> MAAECATQRAPGSVVELLGKSYPQDDHSNLTRKVLTRVGRNLHNQQHHPLWLIKERVKEHFYKQYVGRFGTPLFSVYDNLSPVVTTWQNFDSLLIPADHPSRKKGDNYYLNRTHMLRAHTSAHQWDLLHAGLDAFLVVGDVYRRDQIDSQHYPIFHQLEAVRLFSKHELFAGIKDGESLQLFEQSSRSAHKQETHTMEAVKLVEFDLKQTLTRLMAHLFGDELEIRWVDCYFPFTHPSFEMEINFHGEW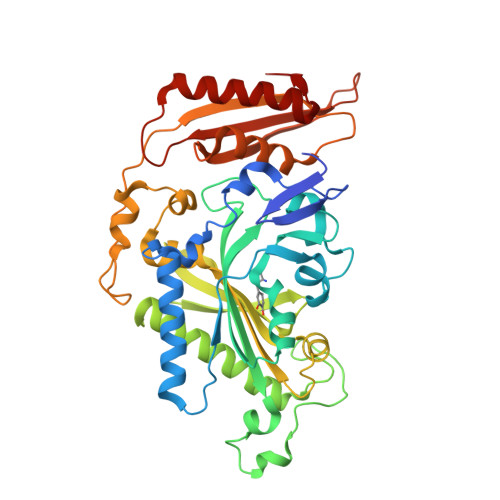LEVLGCGVMEQQLVNSAGAQDRIGWAFGLGLERLAMILYDIPDIRLFWCEDERFLKQFCVSNINQKVKFQPLSKYPAVINDISFWLPSENYAENDFYDLVRTIGGDLVEKVDLIDKFVHPKTHKTSHCYRITYRHMERTLSQREVRHIHQALQEAAVQLLGVEGRF> GSHMCPSGWIPYQERCFYISHTLRSLEESQKYCTSLSSKLAAFDEPSKYYYEVSLPSGLEELLDRSKSYWIQMSKKWRHDYDSQSRYCDKIKKYYQKWKRTFSECAELHPSICESEAFRFPDGIHL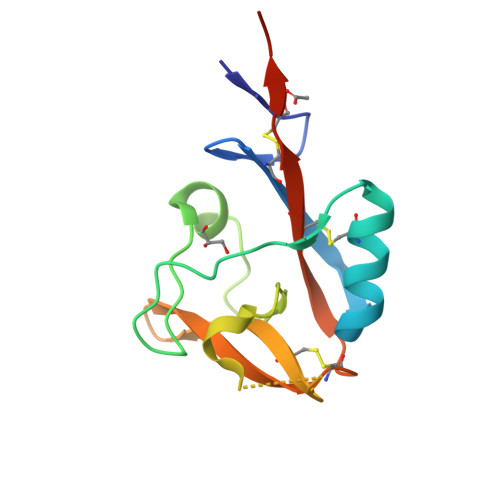N>IVGGKVCPKGECPWQVLLLVNGAQLCGGTLINTIWVVSAAHCFDKIKNWRNLIAVLGEHDLSEHDGDEQSRRVAQVIIPSTYVPGTTNHDIALLRLHQPVVLTDHVVPLCLPERTFSERTLAFVRFSLVSGWGQLLDRGATALELMVLNVPRLMTQDCLQQSRKVGDSPNITEYMFCAGYSDGSKDSCKGDSGGPHATHYRGTWYLTGIVSWGQGCATVGHFGVYTRVSQYIEWLQKLMRSEPRPGVLLRAPFP[2x];>ISYSDGDQCASSPCQNGGSCKDQLQSYICFCLPAFEGRNCETHK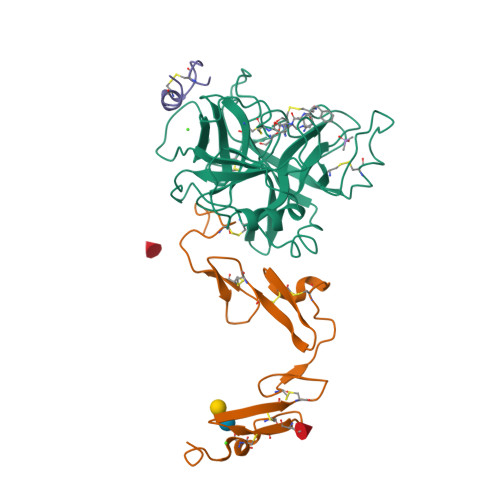DDQLICVNENGGCEQYCSDHTGTKRSCRCHEGYSLLADGVSCTPTVEYPCGKIPILE[2x];>XALCDDPRVDRWYCQFVEGX[2x]>[2x]RCYFRTSSKYGCISNRNLYVFGAVWKTEDCYQCKCKMNAMVCCSLVSIP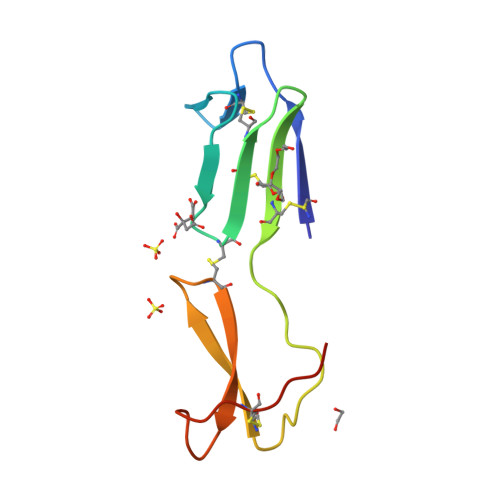KNYDRVNCVGLFHKKSCSIRVVKKTDPDISCKVYNGVG> NNWEQQKKNIEDDLDRYKKRAEELRKEAEKARKEARKTEDPTEEAKKEWEKRCKELEERARKLEDEAKDRVNDLFDSNFFQVIYSGDNDEEEWKKEKDRAEKEIEEWFKRIKEKCEEIKKRLEQ;>SQDASDGLQRLHMLQISYFRDPYHVWYQGNASLGGHLTHVLEGPDTNTTIIQLQPLQEPESWARTQSGLQSYLLQFHGLVRLVHQERTLAFPLTIRCFLGCELPPEGSRAHVFFEVAVNGSSFVSFRPERALWQADTQVTSGVVTFTLQQLNAYNRTRYEL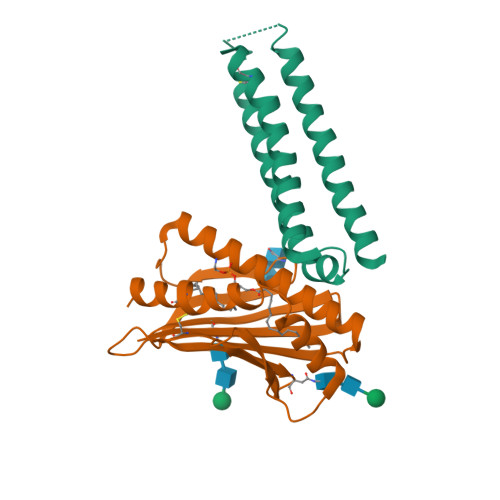REFLEDTCVQYVQKHISAENTKGSQTSRSYTS[2x]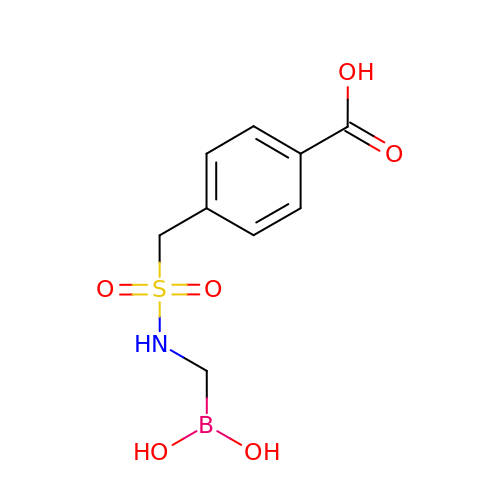4-({[(dihydroxyboranyl)methyl]sulfamoyl}methyl)benzoic acid | C9 H12 B N O6 S | XFGLPAZMEWKDFW-UHFFFAOYSA-N> MDSLSVNQILYPEVHLDSPIVTNKIVAILEYARVPHAYSLEDPTLCQNIKHRLKNGFSNQMIINNVEVGNVIKSKLRSYPAHSHIPYPNCNQDLFNIEDKESTRKIRELLKKGNSLYSKVSDKVFQCLRDTNSRLGLGSELREDIKEKVINLGVYMHSSQWFEPFLFWFTVKTEMRSVIKSQTHTCHRRRHTPVFFTGSSVELLISRDLVAIISKESQHVYYLTFELVLMYCDVIEGRLMTETAMTIDARYTELLGRVRYMWKLIDGFFPALGNPTYQIVAMLEPLSLAYLQLRDITVELRGAFLNHCFTEIHDVLDQNGFSDEGTYHELIEALDYIFITDDIHLTGEIFSFFRSFGHPRLEAVTAAENVRKYMNQPKVIVYETLMKGHAIFCGIIINGYRDRHGGSWPPLTLPLHAADTIRNAQASGDGLTHEQCVDNWKSFAGVKFGCFMPLSLDSDLTMYLKDKALAALQREWDSVYPKEFLRYDPPKGTGSRRLVDVFLNDSSFDPYDVIMYVVSGAYLHDPEFNLSYSLKEKEIKETGRLFAKMTYKMRACQVIAENLISNGIGKYFKDNGMAKDEHDLTKALHTLAVSGVPKDLKESHRGGPVLKTYSRSPVHTSTRNVRAAKGFIGFPQVIRQDQDTDHPENMEAYETVSAFITTDLKKYCLNWRYETISLFAQRLNEIYGLPSFFQWLHKRLETSVLYVSDPHCPPDLDAHIPLYKVPNDQIFIKYPMGGIEGYCQKLWTISTIPYLYLAAYESGVRIASLVQGDNQTIAVTKRVPSTWPYNLKKREAARVTRDYFVILRQRLHDIGHHLKANETIVSSHFFVYSKGIYYDGLLVSQSLKSIARCVFWSETIVDETRAACSNIATTMAKSIERGYDRYLAYSLNVLKVIQQILISLGFTINSTMTRDVVIPLLTNNDLLIRMALLPAPIGGMNYLNMSRLFVRNIGDPVTSSIADLKRMILASLMPEETLHQVMTQQPGDSSFLDWASDPYSANLVCVQSITRLLKNITARFVLIHSPNPMLKGLFHDDSKEEDEGLAAFLMDRHIIVPRAAHEILDHSVTGARESIAGMLDTTKGLIRASMRKGGLTSRVITRLSNYDYEQFRAGMVLLTGRKRNVLIDKESCSVQLARALRSHMWARLARGRPIYGLEVPDVLESMRGHLIRRHETCVICECGSVNYGWFFVPSGCQLDDIDKETSSLRVPYIGSTTDERTDMKLAFVRAPSRSLRSAVRIATVYSWAYGDDDSSWNEAWLLARQRANVSLEELRVITPISTSTNLAHRLRDRSTQVKYSGTSLVRVARYTTISNDNLSFVISDKKVDTNFIYQQGMLLGLGVLETLFRLEKDTGSSNTVLHLHVETDCCVIPMIDHPRIPSSRKLELRAELCTNPLIYDNAPLIDRDATRLYTQSHRRHLVEFVTWSTPQLYHILAKSTALSMIDLVTKFEKDHMNEISALIGDDDINSFITEFLLIEPRLFTIYLGQCAAINWAFDVHYHRPSGKYQMGELLSSFLSRMSKGVFKVLVNALSHPKIYKKFWHCGIIEPIHGPSLDAQNLHTT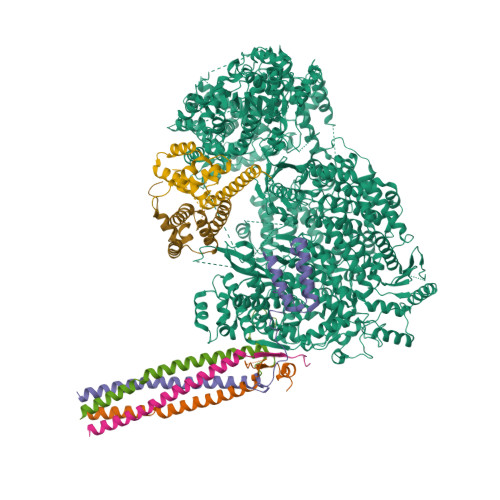VCNMVYTCYMTYLDLLLNEELEEFTFLLCESDEDVVPDRFDNIQAKHLCVLADLYCQPGTCPPIQGLRPVEKCAVLTDHIKAEAMLSPAGSSWNINPIIVDHYSCSLTYLRRGSIKQIRLRVDPGFIFDALAEVNVSQPKIGSNNISNMSIKAFRPPHDDVAKLLKDINTSKHNLPISGGNLANYEIHAFRRIGLNSSACYKAVEISTLIRRCLEPGEDGLFLGEGSGSMLITYKEILKLSKCFYNSGVSANSRSGQRELAPYPSEVGLVEHRMGVGNIVKVLFNGRPEVTWVGSVDCFNFIVSNIPTSSVGFIHSDIETLPDKDTIEKLEELAAILSMALLLGKIGSILVIKLMPFSGDFVQGFISYVGSHYREVNLVYPRYSNFISTESYLVMTDLKANRLMNPEKIKQQIIESSVRTSPGLIGHILSIKQLSCIQAIVGDAVSRGDINPTLKKLTPIEQVLINCGLAINGPKLCKELIHHDVASGQDGLLNSILILYRELARFKDNQRSQQGMFHAYPVLVSSRQRELISRITRKFWGHILLYSGNRKLINKFIQNLKSGYLILDLHQNIFVKNLSKSEKQIIMTGGLKREWVFKVTVKETKEWYKLVGYSALIKD;>MAEEQARHVKNGLECIRALKAEPIGSLAIEEAMAAWSEISDNPGQERATCREEKAGSSGLSKPCLSAIGSTEGGAPRIRGQGPGESDDDAETLGIPPRNLQASSTGLQCHYVYDHSGEAVKGIQDADSIMVQSGLDGDSTLSGGDNESENSDVDIGEPDTEGYAITDRGSAPISMGFRASDVETAEGGEIHELLRLQSRGNNFPKLGKTLNVPPPPDPGRASTSGTPIKKGTDARLASFGTEIASSLTGGATQCARKSPSEPSGPGAPAGNVPECVSNAALIQEWTPESGTTISPRSQNNEEGGDHYDDELFSDVQDIKTALAKIHEDNQKIISKLESLLLLKGEVESIKKQINRQNISISTLEGHLSSIMIAIPGLGKDPNDPTADVEINPDLKPIIGRDSGRALAEVLKKPVASRQLQGMTNGRTSSRGQLLKEFQLKPIGKKMSSAVGFVPDTGPASRSVIRSIIKSSRLEEDRKRYLMTLLDDIKGANDLAKFHQMLMKIIMKSG[4x];>MSKTDWNASGLSRPSPSAHWPSRKLWQHGQKYQTTQDRSEPPAGKRRQAVRVSANHASQQLDQLKAVHLASAVRDLERAMTTLKLWESPQEISRHQALGYSVIMFMITAVKRLRESKMLTLSWFNQALMVIAPSQEETMNLKTAMWILANLIPRDMLSLTGDLLPSLWGSGLLMLKLQKEGRSTSS[2x]> GPHMTGLAAISDALAADLAGLSFSSPVAHVYNPLLYAREPHVAYLSRFGSPPKEVLFVGMNPGPWGMAQTGVPFGEVAVVTEWLGINGTVTRPAGEHPKKRVDGFACRRSEVSGRRLWGFIRERFGTPERFFARFFVANYCPLLFLTAEGGNITPDKLRRGEQEPLFAACDLALRRTVVLLRPRVVIGVGAFAEARCHEALEGFDVE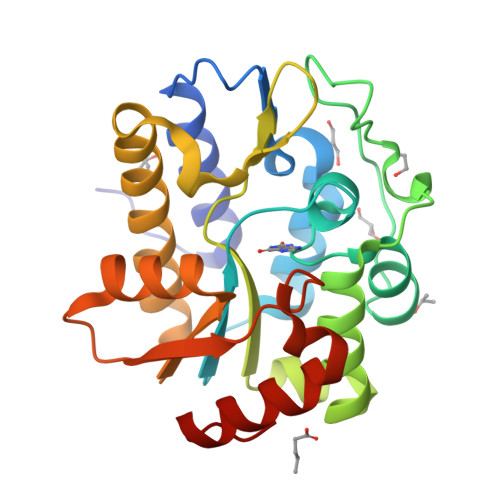VGRIIHPSPASPAANRDWAGTALRQLAELGVDF>HHMLLEFTKMHGLGNDFMVVDLISQRAYLDTATIQRLADRHFGVGFDQLLIVEPPDVPEADFKYRIFNADGSEVEQCGNGVRCFARFVHERHLTNKTNITVQTKAGIVKPELGQNGWVRVNMGYPKFLPNEIPFVAEEPEA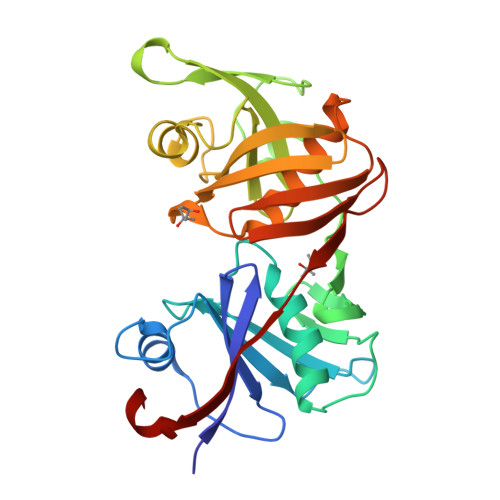LYTLELANDQNISIDVVNMGNPHAVTIVPDVLTADVAGIGPQVESHKRFPERVNAGFMQVIDDKHVRLRVFERGVGETLACGTGACAAAVSGMRRGLLANSVEVELAGGKLQIEWQEGDVVWMTGPTTHVYDGRLDLRYFQ[2x]1,2-DIDECANOYL-SN-GLYCERO-3-PHOSPHOCHOLINE 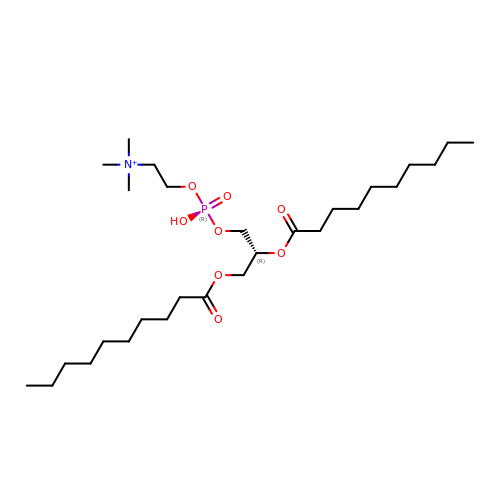| C28 H57 N O8 P | MLKLDGSYMHFAOC-AREMUKBSSA-O2-methyl-3-[(1R)-1-{[4-methyl-7-(morpholin-4-yl)pyrido[3,4-d]pyridazin-1-yl]amino}ethyl]benzonitrile 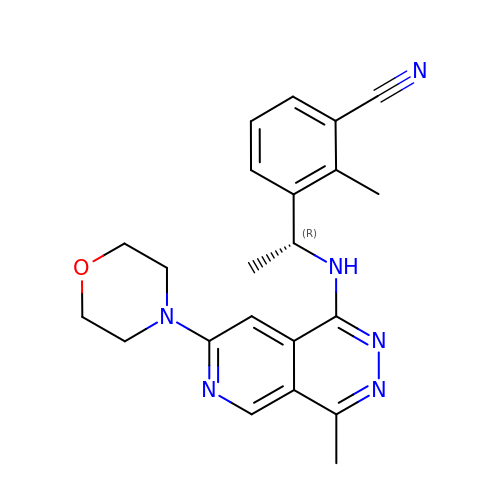| C22 H24 N6 O | ILPWEAHQRAWJIU-OAHLLOKOSA-N>[4x]SNAMKRKVQVKNITIGEGRPKICVPIIGKNKKDIIKEAKELKDACLDIIEWRVDFFENVENIKEVKEVLYELRSYIHDIPLLFTFRSVVEGGEKLISRDYYTTLNKEISNTGLVDLIDVELFMGDEVIDEVVNFAHKKEVK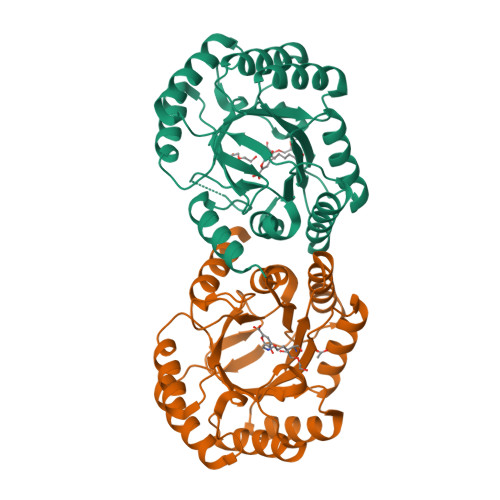VIISNHDFNKTPKKEEIVSRLCRMQELGADLPKIAVMPQNEKDVLVLLEATNEMFKIYADRPIITMSMSGMGVISRLCGEIFGSALTFGAAKSVSAPGQISFKELNSVLNLLHKSIN> KPKLLNKFDKTIKAELDAAEKLRKRGKIEEAVNAFKELVRKYPQSPRARYGKAQCEDDLAEKRRSNEVLRGAIETYQEVASLPDVPADLLKLSLKRRSDRQQFLGHMRGSLLTLQRLVQLFPNDTSLKNDLGVGYLLIGDNDNAKKVYEEVLSVTPNDGFAKVHYGFILKAQNKIAESIPYLKEGIESGDPGTDDGRFYFHLGDAMQRVGNKEAYKWYELGHKRGHFASVWQRSLYNVNGLKAQPWWTPKETGYTELVKSLERNWKLIRDEGLAVMDKAKGLFLPEDENLREKGDWSQFTLWQQGRRNENACKGAPKTCTLLEKFPETTGCRRGQIKYSIMHPGTHVWPHTGPTNCRLRMHLGLVIPKEGCKIRCANETKTWEEGKVLIFDDSFEHEVWQDASSFRLIFIVDVWHPELTPQQRRSLPAI;> DGDQCETSPCQNQGKCKDGLGEYTCTCLEGFEGKNCELF

Here, we report crystallographic and biochemical results on the structure and substrate selectivity of AspH. The results reveal a key role for the TPR domain of AspH in substrate binding and, unexpectedly, that the preferred EGFD-substrates of AspH have a non-canonical (Cys3–4) disulfide pattern. Whilst the oxygenase domain fold of AspH is typical for the 2OG oxygenase superfamily, details of its active site and the role of the TPR domain in EGFD-substrate binding are remarkable. Whatever the precise extent of conformational changes during catalysis, the results reveal a central role for the TPR domain in enabling AspH catalysis—without it, 2OG turnover occurs, but EGFDs are not hydroxylated.

AspH-TPR-Ox was successfully co-crystallized with a 39-residue fragment of hFX EGF1 (AspH-TPR-Ox:hFX). The AspH-TPR-Ox structure reveals electron density at the active site corresponding to 18 of the 39 hFX EGF1 substrate residues (aa 99–116: -GKC3KDGLGEYTC4TC5LEGF-) and for a disulfide linkage between Cys101hFX and Cys110hFX. The N-terminal region of hFX (aa 100–105) interacts with the AspH-Ox domain and the C-terminal region of hFX (aa 106–116) interacts with the TPR domain. Comparison of AspH structures with and without substrate implies that induced fit involving substantial conformational changes during formation of the AspH-TPR-Ox:hFX protein:protein complex occurs; the distance between Leu433 on repeat 3 of the TPR domain to Pro756 of the oxygenase domain near the C-terminus is reduced from 20 to ~14 Å on substrate binding. The side chain of Asp103hFX, the substrate asparagine undergoing hydroxylation, is at the i+2 position of a Type I β-turn adjacent to the active site metal and was modelled in two conformations, both of which are positioned to form salt bridges with the side chains of Arg688 and Lys666. The Asp103hFX carboxylate side chain in conformation A is positioned to form a hydrogen bond (3.2 Å) with the side chain of Gln627, whilst in conformation B the carboxylate is positioned to interact with the active site metal (2.6 Å) trans to His725. Asp103hFX conformation A is poised for C-3 hydroxylation such that its pro-3R-hydrogen projects towards the metal (Cβ-metal distance ~4.5 Å), consistent with reported (3R)-stereoselectivity for AspH catalysis. Notably, the highly-conserved hFX tyrosine, Tyr108hFX, that is part of the consensus EGFD sequence for AspH hydroxylation, binds in a mostly hydrophobic pocket located between TPR repeats 5 and 6 located on the concave surface of the TPR domain. Unexpectedly, in the AspH-TPR-Ox substrate complex we observed a non-canonical disulfide bridge, i.e. between Cys101hFX and Cys110hFX for the hFX substrate, in effect forming a ten-residue ring. The observed hFX disulfide corresponds to a non-canonical Cys3–4 EGFD disulfide link, suggesting this pattern is required for AspH catalysis rather than the established (Cys1–3, 2–4, 5–6) disulfide pattern.>MSTPNSYDDEELEELLRRKAAQEQKRIEEERKRKAELESQKES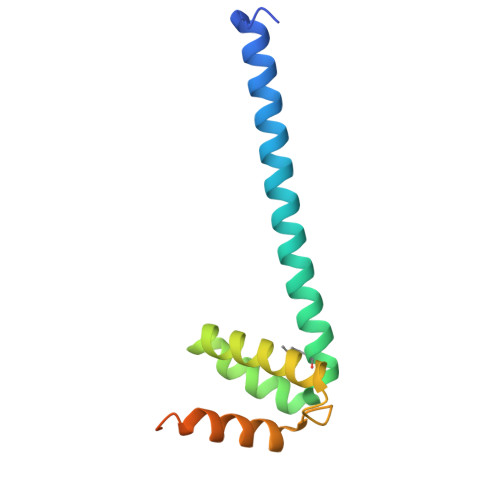IMRVILTPEARQRLTNIKLVKPEFAESLENQLIALAQSGRIKIPITDEELKQILEQISQQNRRDFKIQIRERGWKHHHHHH[2x]>MDLTVEPNLHSLITSTTHKWIFVGGKGGVGKTTSSCSIAIQMALSQPNKQFLLISTDPAHNLSDAFGEKFGKDARKVTGMNNLSCMEIDPSAALKDMNDMAVSRANNNGSDGQGDDLGSLLQGGALADLTGSIPGIDEALSFMEVMKHIKRQEQGEGETFDTVIFDTAPTGHTLRFLQLPNTLSKLLEKFGEITNKLGPMLNSFMGAGNVDISGKLNELKANVETIRQQFTDPDLTTFVCVCISEFLSLYETERLIQELISYDMDVNSIIVNQLLFAENDQEHNCKRCQARWKMQKKYLDQIDELYEDFHVVKMPLCAGEIRGLNNLTKFSQFLNKEYNPITDGKVIYELEDKELEHHHHHH[3x];>[2x]MKHHHHHHPMGSELTEAEKRRLLRERRQKKFSNGGAS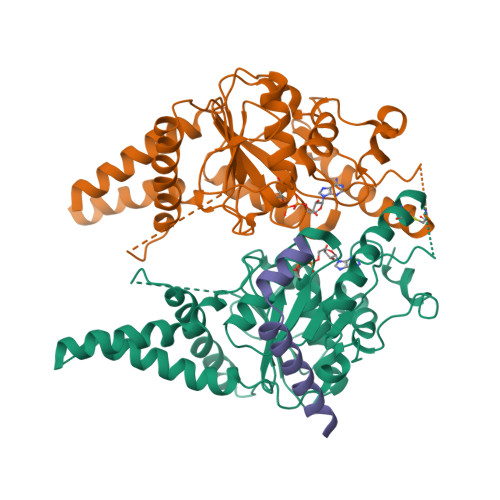SRLNKITGW>MKWTRSVKVPFPSVWHRFQAKDLTSQQLVWYRVQDLPEDRFEDAIRHMCDYFARDELMNQAKGLAKDLVAMGDVVALWKAMLPDRMSLVCFREGSDEIVGVNILDVASRSDKDNAQFNSAIFQAIYDTIEYVSHQANIFDRYNVDHYLNAMGLSVDP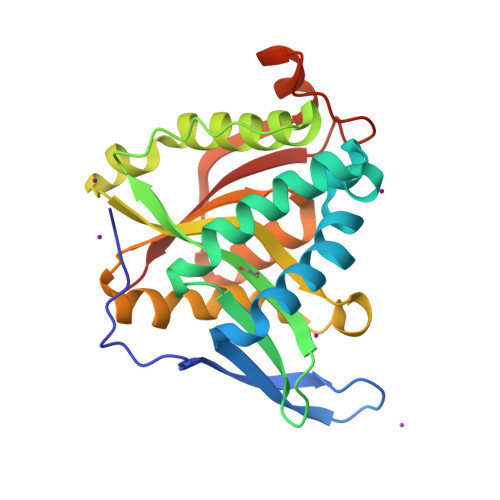KYRGRGIATEILRARIPLCRAVGLKLSATCFTGPNSQTAATRVGFQEDFTITYGELARVDQRFNYPGIEENFCKYMSLRVD[4x]(2S)-2-{6'-[(6-aminopyridin-3-yl)sulfonyl]-2'-(phenylamino)-2,3'-bipyridin-5-yl}-1,1,1-trifluoropropan-2-ol 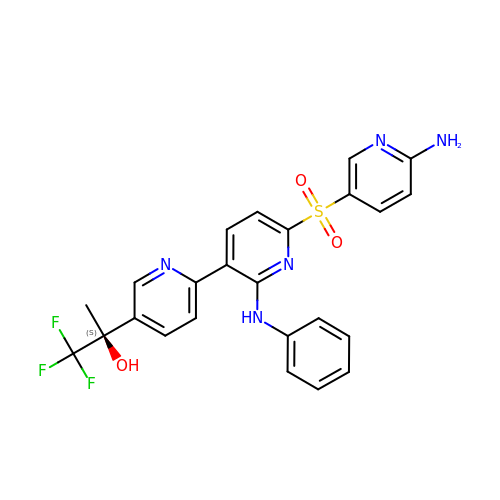| C24 H20 F3 N5 O3 S | LJCXNEAHAINFGA-QHCPKHFHSA-N>MSGMEKVTVVLYVNGDEVALVHAFMTTASLLAKEGKLVEKLILTSNFTERTVRRAFDLVRELLPAKA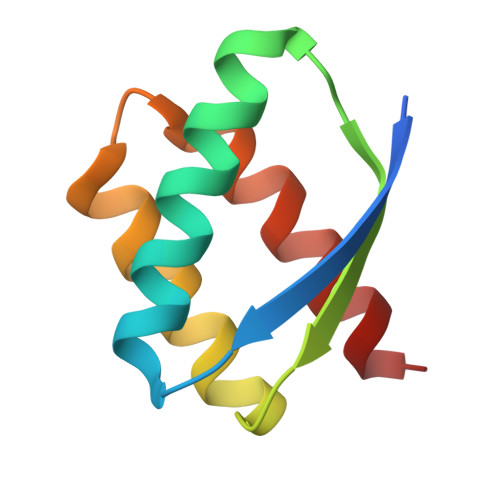EIIDALREEAEKYFAE[2x]Dodecahedron-base is a small icosahedral virus-like particle composed of 12 copies of the Ad3 pentameric Pb protein and is capable of efficient cell entry. Virus-like particles, called dodecahedron-fiber (DF), are generated during the adenovirus serotype 3 (Ad3) life cycle in infected cells. These symmetrical, dodecahedral particles are composed of 12 copies of the viral penton complex, which comprises the pentameric penton base (Pb) and the attached trimeric fiber, both of which are essential for viral cell entry. Through careful examination of the crystal structure, it was determined that residues 48–61 of Ad3 Pb, the Dd building blocks, interlock within the particle through strand-swapping. The strand-swapping considerably increases the contacts between neighboring Pb pentamers which otherwise associates only through three small loop regions.

The atomic structure of the Ad3 Dd was first determined using crystals of space group P213 in which there are 20 Pb monomers, i.e. 1/3 of the Dd, in the asymmetric unit. The structure was solved by molecular replacement using a model derived from the Ad2 Dd crystal structure and refined with an Rfree = 0.290 at a resolution of 4.75 Å. The overall fold of the Ad3 Pb molecule is very similar to that of Ad2. Structural differences concern principally the variable loop, which is longer than in Ad2 but relatively well ordered. A second loop region containing the internalization motif RGD (hereafter called the RGD loop) is only partially visible in the Ad3 structure and rather poorly ordered. It is possible that the loop is proteolyzed in the crystal as N-terminal sequencing and mass spectrometry of Dd preparations often indicated the absence of residues 313 to 347 (data not shown). In both Ad3 Dd crystal forms, the visible electron density for the Pb peptide chain starts at residue Pro48, while a very strong positive electron density (>10 σ and >18 σ, respectively for each crystal form) is consistently present in averaged Fo-Fc maps on the Pb 5-fold axis and coordinated by Glu451 from each subunit. As Ca2+ was present during the crystallization, it is most likely that this density corresponds to a bound calcium ion. However, during refinement of the Ad3 model based on the Ad2 Pb structure it became obvious that there was an interruption of the peptide chain between residues 59 to 62, and Fo-Fc and 2Fo-Fc electron density maps suggested an alternative trace. This trace corresponds to an exchange of the N-terminal residues 48–61 between monomers related by a 2-fold axis of the dodecahedron.

> MRRRAVLGGAVVYPEGPPPSYESVMQQQAAMIQPPLEAPFVPPRYLAPTEGRNSIRYSELSPLYDTTKLYLVDNKSADIASLNYQNDHSNFLTTVVQNNDFTPTEASTQTINFDERSRWGGQLKTIMHTNMPNVNEYMFSNKFKARVMVSRKAPEGVTVNDTYDHKEDILKYEWFEFILPEGNFSATMTIDLMNNAIIDNYLEIGRQNGVLESDIGVKFDTRNFRLGWDPETKLIMPGVYTYEAFHPDIVLLPGCGVDFTESRLSNLLGIRKRHPFQEGFKIMYEDLEGGNIPALLDVTAYEESKKDTTTETTTKKELKIQPLEKDSKSRSYNVLEDKINTAYRSWYLSYNYGNPEKGIRSWTLLTTSDVTCGAEQVYWSLPDMMQDPVTFRSTRQVNNYPVVGAELMPVFSKSFYNEQAVYSQQLRQATSLTHVFNRFPENQILIRPPAPTITTVSENVPALTDHGTLPLRSSIRGVQRVTVTDARRRTCPYVYKALGIVAPRVLSSR The re-acylation is catalyzed by lysophosphatidylcholine acyltransferase (LPCAT) and among the four LPCAT members in human, the LPCAT3 preferentially introduces polyunsaturated acyl onto the sn-2 position of lysophosphatidylcholine, thereby modulating the membrane fluidity and membrane protein functions therein. Combining the x-ray crystallography and the cryo-electron microscopy, we determined the structures of LPCAT3 in apo-, acyl donor-bound, and acyl receptor-bound states. A reaction chamber was revealed in the LPCAT3 structure where the lysophosphatidylcholine and arachidonoyl-CoA were positioned in two tunnels connected near to the catalytic center. The structural and functional analysis provides the basis for the re-acylation of lysophosphatidylcholine and the substrate preference during the reactions.

After solubilization with LMNG, the oligomeric LPCAT3 was further separated from its monomers by size-exclusion chromatography in glyco-diosgenin (GDN) supplemented with 0.2 mM arachidonoyl CoA. The 3D refinement using C2 symmetry generated an EM density map with an overall resolution of 3.49 Å and a resolution of about 3 Å at the core region of cLPCAT3 protomers. The cytoplasmic end of the vertical tunnel is lined with positively charged amino acids and thereby provides a docking surface for the coenzyme A moiety, where the binding of CoA is stabilized by the electrostatic interactions among the pyrophosphate section of CoA and basic residues R409, as well as K365, 368, and 373. The araCoA extends into the T-shape chamber and turns at the joint point near H388 to a “side pocket” with its double-bonds in the acyl chain, and the carbonyl oxygen of the arachidonoyl pointing to the conserved residue N352, implying its role as protonation reagent in the hydrolysis of thioester bond. When N352 was mutated, the cLPCAT3 show an impaired acyltransferase activity, confirming its critical role in the reaction. To hold the acyl chain, the side pocket is in general lined with hydrophobic residues, e.g., F344, I348, I404, M446, and L450, and the functional assay showed that the mutations on those sites could reduce the enzymatic activities to various degrees. Unexpectedly, the E401A mutation fully abolished the acyltransferase activity, implying the importance of E401 in maintaining the binding of the acyl-CoA molecule. The cryo-EM map analysis on cLPCAT3/araCoA revealed the non-protein electron density sandwiched by cLPCAT3 protomers and two 1,2-dioleoyl-sn-glycero-3-phosphocholine (DOPC) molecules were well modeled into the large blobs of electron density. This non-contact dimerization might be mediated by those intermediary lipid molecules and the relatively harsh detergents used in the crystallization trial deprived the cLPCAT3 of the lipids bound, resulting in the monomeric biological unit in cLPCAT3 crystals.

>MGAERDESGAGAAVLVPLLGFGSNRPAGPAEKMAVAGSGWSLARVAEALGSSEQALRLIVSILMGYPFALFQRYFLFQKETYLIHLYNVFTGLSIAYFNFGMQFFHSLLCVLIQFLILRLMGRTVTAVFTTFVFQMTYLMAGYYFTATEHYDIKWTMPHCVLTLKLIGLAIDYYDGGKDPELLTPEQRRFAVRGVPTLLEVSGFSYFYGAFMVGPQFSMTDYQKLAKGEMTDVPGQRPNSFVPALKRLSLGLLFLVTYTLSSPYISEEYLISDDYMEKPFWFRCGYILVWGKIILYKYVTCWLVTEGVCILVGLGYNGNDQNGKPVWDACANMKVWLYETTPLFTGTIASFNINTNAWVARYVFKRLKFLGNKLLSQALALFFLAIWHGLHSGYLVCFQMELLIVIVERQVINLVRDSPTLSTLASITALQPIFYVLQQTNHWMFMGYSLVPFCLFTWDKWMKVYKSIYFLGHVLFFTLLLVLPYIRKLLVPRKEKLKKAE[2x]> QEFHFGPCQVKGVVPQKLWEAFWAVKDTMQAQDQITSARLLQQEVLQQVSDA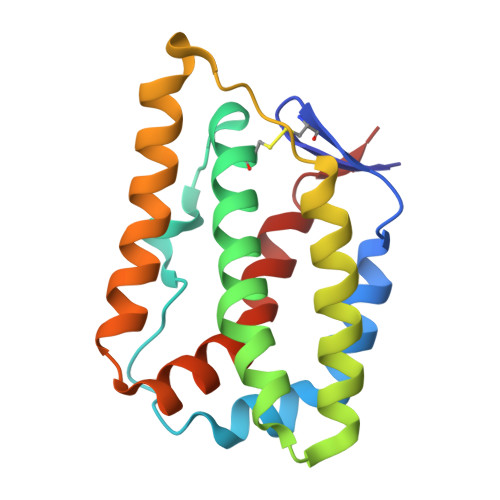ESCYLVHTLLEFYLKTVFKNHHQRTVEVRTLKSFSTLANNFVLIVSQLQPSQENEMFSIRDSAHRRFLLFRRAFKQLDVEAALTKALGEVDILLTWMQKFYKL>[2x]GSHESYTLTPEVGELIEKVRKAHQETFPALCQLGKYTTNNSSEQRVSLDIDLW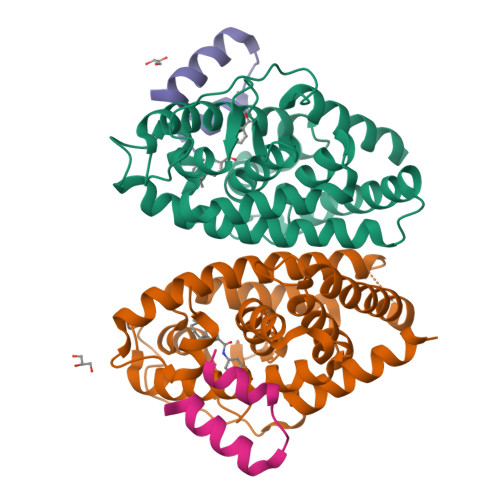DKFSELSTKCIIKTVEFAKQLPGFTTLTIADQITLLKAACLDILILRICTRYTPEQDTMTFSDGLTLNRTQMHNAGFGPLTDLVFAFANQLLPLEMDDAETGLLSAICLICGDRQDLEQPDRVDMLQEPLLEALKVYVRKRRPSRPHMFPKMLMKITDLRSISAKGAERVITLKMEIPGSMPPLIQEMLENSEGLD;>KHKILHRLLQDSSSPVDLAKLTAEATGK[2x]>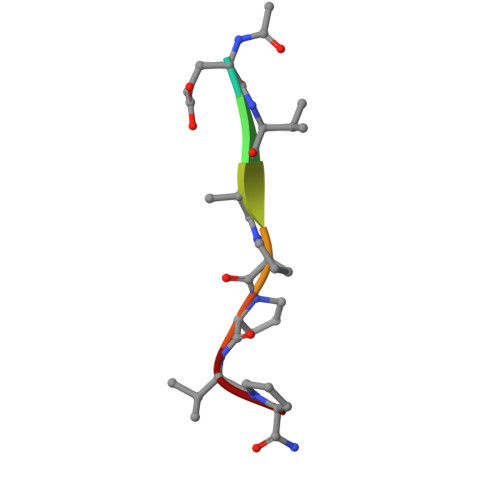 XEVAPPVP> METITMTLVQEPELFLECYSVTPDLFAGKSLAEIADLPAHEGKIQWKLGDFFKFEGKAGETAADTKIVVNGNVRRMKRFGQQMTAGEIIINSDADMYIGGWMKGGKITVKGNADSFLG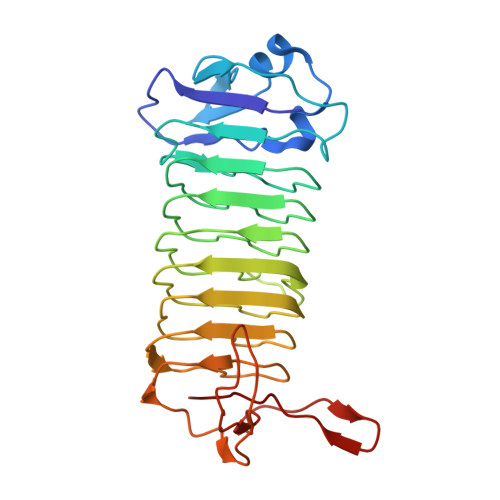IAMEGGEILIEGDAQNHVGSAYRGDWRGMSGGLIRVKGKAGNDIGTAMTGGTIIIEGDAFIHVLTHAEGGTVIIKGDVEGRVGGQMVKGDAYILGNLLYPLPGFKKVATVEKEVDGATYTFDQFIGDLGERKEKKKGEIIYGNIFLKK>[2x]MEKKDLIIRVAGEGGEGIISSGDFIAAACARAGLEVYTFKTFPAEIKGGYAMYQVRASSEKLYCQGDTFDVFCAFNGEAYEQNKDKIKPGTAFVYDYPGGDFEPDEIPEGVFAYPIPMSQTAKEMKSYRSKNMVALGALSELFNISENTLKEVLSDKFGKKGEEVLAFNLEAFDKGKALAKALTKADPFRVADPQEPKDVIIMAGNDAVGLGGILGGLEFFSAYPITPATEVAKYVATHLPKCGGDLVQAEDEIASIAQVLGASYAGKKSMTATSGPGLALMSEMLGMAHMSETPCLVVDVQRGGPSTGLPTKHEQSDLFLAIHGGHGDSPRIVLSVEDVKDCISMTVDGLNLAEKYQAPVIVL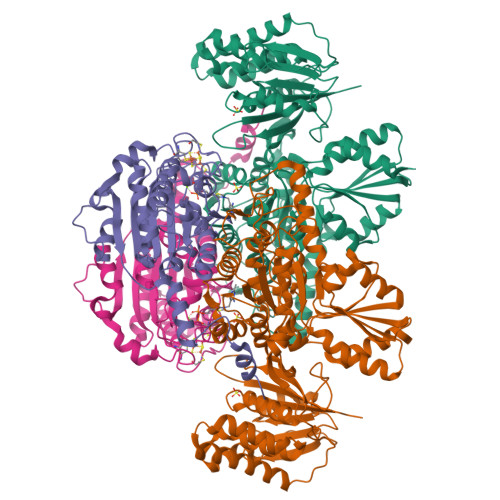SDGSLAFSTQTIPRPKPEDFTIINRKTWDGQGTYKRYELTEDNISPMAAPGTPNAKHIATGLEHGETGAPNYSPANHELMHRKRFNKQNSVLDFYKNMEVEGVEGEADVGIITWGSTIGVVREAMQRLTAEGLKVKAMYPKLLWPMPVADYDAFGATCKKVIVPEVNFQGQLSHFIRAETSIKPIPYTICGGLPFTPEMIVNRVKEEIQ;>[2x]MTVEAFHKMENMKPKDYKSEVPTTWCPGCGHFGILNGVYRAMAELGIDSTKFAAISGIGCSSRMPYFVDSYKMHTLHGRAGAVATGTQVARPDLCVVVAGGDGDGFSIGGGHMPHMARKNVNMTYVLMDNGIYGLTKGQYSPTSRPEMTAYTTPYGGPENPMNPLLYMLTYGATYVAQAFAGKPKDCAELIKGAMEHEGFAYVNIFSQCPTFNKIDTVDFYRDLVEPIPEDHDTSDLGAAMELARRPGGKAPTGLLYKTSAPTLDQNLAKIRERLGGHVGYDKNKIIALAKP> MFDQLAVFTPQGQVLYQYNCLGKKFSEIQINSFISQLITSPVTRKESVANANTDGFDFNLLT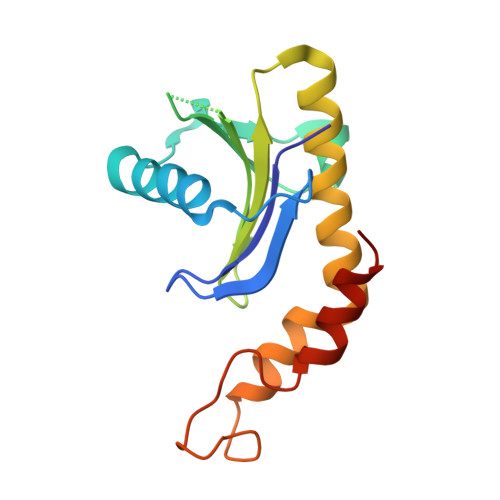INSEHKNSPSFNALFYLNKQPELYFVVTFAEQTLELNQETQQTLALVLKLWNSLHLSESILKNRQGQNEKNKHNYVDILQGIEDDLKKFEQYFRIK>GPLGSMVTEQEVDAIGQTLVDPKQPLQARFRALFTLRGLGGPGAIAWISQAFDDDSALLKHELAYCLGQMQDARAIPMLVDVLQDTRQEPMVRHEAGEALGAIGDPEVLEILKQYSSDPVIEVAETCQLAVRRLEWLQQHGGEPAAGPYLSVDPAPPAEERDV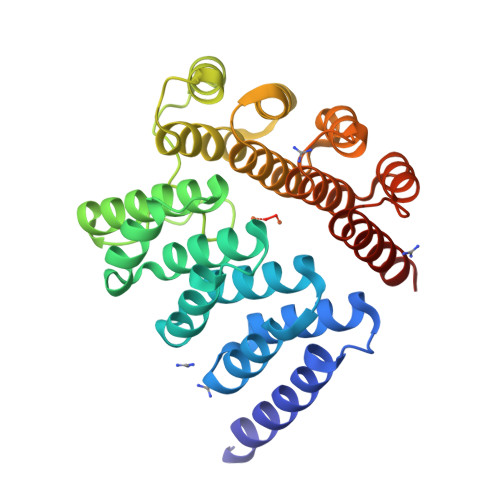GRLREALLDESRPLFERYRAMFALRNAGGEEAALALAEGLHCGSALFRHEVGYVLGQLQHEAAVPQLAAALARCTENPMVRHECAEALGAIARPACLAALQAHADDPERVVRESCEVALDMYEHETGRAFQ[2x]> QAKHKQRKRLKSSCKRHPLYVDFSDVGWNDWIVAPPGYHAFYCHGECPFPLADHLNSTNHAIVQTLVNSVNSKIPKACCVPTELSAISMLYLDENEKVVKKDYQDMVVEGCGCR;> QNLDSMLHGTGMKSDSDQKKSENGVTLAPEDTLPFLKCYCSGHCPDDAINNTCITNGHCFAIIEEDDQGETTLASGCMKYEGSDFQCKDSPKAQLRRTIECCRTNLCNQYLQPTLPPVVIGPFFDGSIR;> SGRGEAETRECIYYNANWELERTNQSGLERCEGEQDKRLHCYASWRNSSGTIELVKKGCWLDDFNCYDRQECVATEENPQVYFCCCEGNFCNERFTHLP

Bone morphogenetic proteins (BMPs) and other members of the transforming growth factor-β (TGF-β) superfamily, like the activins, growth and differentiation factors (GDFs) and TGF-βs are secreted signaling proteins that regulate the development, maintenance and regeneration of tissues and organs. Members of the TGF-β superfamily bind two different types of serine/threonine-kinase receptors termed type I and type II receptors. In the present study we analyze the interaction of BMP-2 with its type I receptor BMPR-IA and its type II receptor ActR-IIB. ActR-II and ActR-IIB bind activin A (Act-A) with high affinity in the low nanomolar range leading to activation of the SMAD-2/-3 pathway, whereas binding of BMP-2 occurs with low-affinity in the micromolar range resulting in the activation of the SMAD-1/-5/-8 pathway.

Crystals from this complex comprising the BMP-2 variant L100K/N102D were obtained under different crystallization conditions and exhibit distinct morphology. Analysis of this complex yielded a hexameric ligand-receptor arrangement with all receptor binding epitopes occupied as expected for the dimeric BMP-2. Inspection of the receptor-ligand interactions of both BMP-2/receptor complexes (comprising BMP-2 L100K/N102D, in the following termed ternary complex (1:2:2), or wildtype BMP-2, in the following termed ternary complex (1:1:1)) demonstrates that the ligand-receptor interfaces are highly similar. The BMP-2 double variant L100K/N102D binds to ActR-IIB with an affinity (KD ~ 140 nM) almost as high as for the interaction of Act-A with ActR-IIB (KD ~ 60 nM). Confirming this, our structure of the ternary complex (1:2:2) comprising BMP-2L100K/N102D shows no additional intermolecular H-bond between the lysine side chain and Cys59 of ActR-IIB. In the structures of the Act-A:ActR-IIBECD and the ternary complex (1:2:2) of BMP-2L100K/N102D the Lys and Asp residues form a stable intramolecular salt bridge. Accordingly, Lys100 and Asp102 (in BMP-2L100K/N102D) exhibit low temperature factors indicating that both residues are quite immobile. The "rigid lid" centered above the conserved H-bond between BMP-2 Ser88 Oγ and ActR-IIB Leu61 amide might provide an effective shielding from solvent access thereby enhancing the strength of this particular H-bond. The double variant L100K/N102D shows a large increase in affinity for ActR-IIB, in addition the affinity for ActR-II is moderately increased (threefold), but binding to BMPR-II remains unaltered.>[2x]CC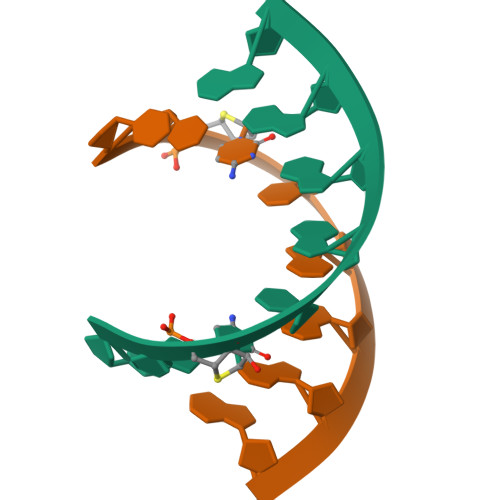CCGGGG> GSHMIASLSDSVSNAREERMALRQEQEQLQSRIQSLMQRAPVWLAAQNSLNQLSEQCGEEFTSSQDVTEYLQQLLEREREAIVERDEVGARKNAVDEEIERLSQPGGSEDQRLNALAERFGGVLLSEIYDDVSLEDAPYFSALYGPSRHAIVVPDLSQVTEHLEGLTDCPEDLYLIEGDPQSFDDSVFSVDELEKAVVVKIADRQWRYSRFPEVPLFGRAARESRIESLHAEREVLSERFATLSFDVQKTQRLHQAFSRFIGSHLAVAFESDPEAEIRQLNSRR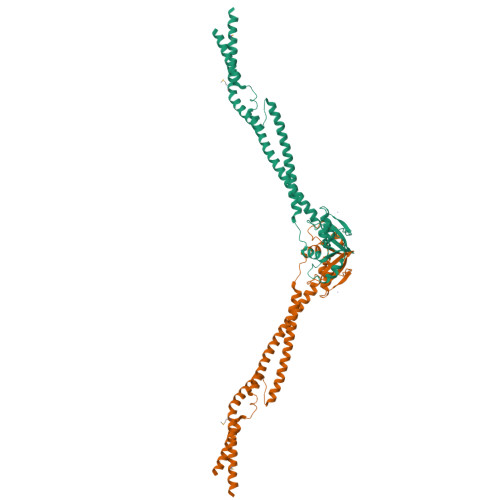VELERALSNHENDNQQQR>[4x]MQFPQLDPATLAAFSAAFRGELIWPSDADYDEARRIWNGTIDRRPALIARCTSTPDVVAAVSFARKSGLLVAVRGGGHSMAGHSVCDGGIVIDLSLMNSIKVSRRLRRARAQGGCLLGAFDTATQAHMLATPAGVVSHVGLGGLVLGGGFGWLSRKY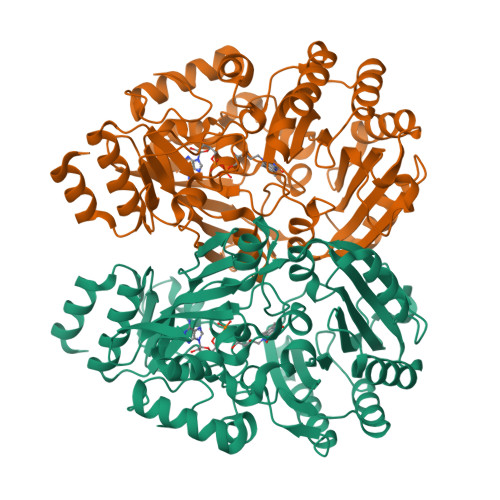GLSIDNLTSVEIVTADGGVLTASDTENPDLFWAVRGGGGNFGVVTAFEFDLHRVGPVRFASTYYSLDEGPQVIRAWRDHMATAPDELTWALYLRLAPPLPELPADMHGKPVICAMSCWIGDPHEGERQLESILHAGKPHGLTKATLPYRALQAYSFPGAVVPDRIYTKSGYLNELSDEATDTVLEHAADIASPFTQLELLYLGGAVARVPDDATAYPNRQSPFVTNLAAAWMDPTEDARHTAWAREGYRALAGHLSGGYVNFMNPGEADRTREAYGAAKFERLQGVKAKYDPTNLFRLNQNIPPSSP Interestingly, PMX is a multitargeted antifolate that also inhibits the folate-dependent reactions catalyzed by glycinamide ribonucleotide (GAR) formyltransferase (GARFTase) (in the trifunctional GARFTase/glycinamide ribonucleotide synthase (GARS)/aminoimidazole ribonucleotide synthetase (AIRS) enzyme) and 5-aminoimidazole-4-carboxamide ribonucleotide formyltransferase (AICARFTase) (in the bifunctional enzyme AICARFTase/inosine monophosphate cyclohydrolase (ATIC)) in de novo purine biosynthesis. Although all these antifolates are used clinically, their use is often associated with dose-limiting toxicities arising from the lack of tumor selectivity, as well as emergence of drug resistance. By metabolite rescue in KB cells and in vitro enzyme assays, de novo purine biosynthesis was identified as a targeted pathway (at 5-aminoimidazole-4-carboxamide ribonucleotide formyltransferase (AICARFTase) and glycinamide ribonucleotide formyltransferase (GARFTase)). To better understand the molecular effects of modifications to 6-substituted thieno[2,3-d]pyrimidine analogs on GARFTase inhibition, we determined the structures of select analogs (4, 5, 9, and 10) with a range of inhibitor potencies in complex with GARFTase and β-GAR substrate. The thieno[2,3-d]pyrimidine scaffold of all analogs makes polar contacts with the backbone atoms of Leu899, Glu948, and Asp951 in GARFTase.

Thus, in addition to replacing the 1′,4′-phenyl ring by a 2′,5′-pyridyl ring in compound 4, we introduced an ortho fluorine in the 2′,5′-pyridyl ring to afford compound 5. Compound 5, a fluorinated analog of the noninhibitor 4, shows modest inhibition with a Ki = 13.7 μM, implying that intramolecular conformational stabilization occurs with the pyridine N···H–N that positions 5 to bind to GARFTase. Compound 5 harbors the same polar contacts between GARFTase and its l-glutamate as 9 and 10, and the pyridine N of 5 now forms the intramolecular contacts with the amide NH, as indicated in the crystal structure. Taken together, our comparative analysis of the crystal structures of the fluorinated compounds 9 and 5 versus related des-fluorinated compounds 4 and 10 provides molecular details in the solid state, which account for the dramatic increase in potency in one case where an intramolecular fluoro-hydrogen contact may be important and another in which an intramolecular pyridine N-hydrogen contact with the amide NH is necessary. Both intramolecular bonds in 9 and 5 restrict the conformation and are clearly important for GARFTase inhibition. The presence of a fluoro-amide hydrogen contact and a pyridine-amide NH contact was corroborated by NMR and was also seen in the crystal structure of GARFTase in complex with compounds 9 and 5, respectively. For compounds 5, 8, 10, and 11, adenosine was completely protective, establishing de novo purine biosynthesis as the targeted pathway. Neither compounds 5 and 1 nor MTX inhibited ATIC up to 200 μM.

> MARVAVLISGTGSNLQALIDSTREPNSSAQIDIVISNKAAVAGLDKAERAGIPTRVINHKLYKNRVEFDSAIDLVLEEFSIDIVCLAGFMRILSGPFVAKWNGKMLNIHPSLLPSFKGSNAHEQALETGVTVTGCTVHFVAEDVDAGQIILQEAVPVKRGDTVATLSERVKLAEHKIFPAALQLVASGTVQLGENGKICWVKEEHHHHHH> MDKDEAWKQVEQLRREGATRIAYRSDDWRDLKEAWKKGADILIVDASRLREAADAARAAGEATGDEELIAKAEAYRDEAWKQVEQLRREGATEIAYRSDDWRDLKEAWKKGADILIVDGLRRGRIARELERLAKEEGDPALLAAAEAAREAAWKQVEQLRREGATRIAYRSDDWRDLKEAWKKGADILIVDNRARLRRAEEEVAETGDPDNEELIRETRERAREEGWKQVEQLRREGATEIAYRSDDWRDLKEAWKKGADILIVDATLEHHHHHH

In this work, we diversified a de novo TIM barrel by extending multiple βα‐loops using constrained hallucination. For the diversification experiment, we used the de novo TIM barrel sTIM11‐SB as the base scaffold. This variant contains a stabilizing salt bridge cluster in the lower part of the β‐barrel (Kordes et al., 2022). Here, we introduced two or three helical insertions into minimal loops in the de novo designed TIM barrel sTIM11‐SB.

In the case of HalluTIM3‐1, the crystal structure shows all three intended hallucinated extensions in their entirety, verifying their successful incorporation into sTIM11‐SB. One minor deviation between HalluTIM3‐1 and the base scaffold is observed within the N‐terminal α‐helix of the barrel, as these residues do not form a continuous α‐helix. In the case of HalluTIM3‐1, the crystal has an uncommonly high solvent content of 78% (Matthews coefficient: 5.6), that may influence the quality of the data and in combination with a certain flexibility of the extensions, lead to the rather noisy diffraction data. Upon comparison of the obtained crystal structures to corresponding structure predictions using ColabFold, we observed an accurate prediction for HalluTIM2‐2 with a root mean square deviation (RMSD) over all Cα atoms of about 1.2 Å but found major differences in the case of HalluTIM3‐1 as the RMSD over all Cα atoms is over 4.1 Å. These discrepancies are mainly due to the different angles of the extensions from the barrel core, especially for insertion 1 that does not form a continuous α‐helix. The structure prediction shows straighter extensions, whereas two of the extensions in the crystal structure tilt more to the outside. When comparing each individual extension with the corresponding prediction, we observe accurate predictions below 1.0 Å RMSD except for the first extension of HalluTIM3‐1, which shows a higher deviation with 2.34 Å. For HalluTIM3‐1, where the crystal structure and prediction differ, we obtained varying qualities of the fits. The theoretical scattering curve of the predicted structure shows a high χ 2 of 8.9, whereas the crystal structure matches the experimental data with a significantly lower χ 2 of 2.0, indicating that the crystal structure matches the protein in solution more closely. In contrast, in HalluTIM2‐2 and HalluTIM3‐1, a major pocket is formed through the introduced fragments above the C‐terminal end of the inner β‐sheet. These pockets show differences in size with pocket volumes of 1006 Å3 in HalluTIM3‐1 and 2000 Å3 in HalluTIM2‐2.> AEFASGSGQSTRYWDCCKPSCAWPGKAAVSQPVYACDANFQRLSDFNVQSGCNGGSAYSCADQTPWAVNDNLAYGFAATSIAGGSESSWCCACYALTFTSGPVAGKTMVVQSTSTGGDLGSNQFDIAMPGGGVGIFNGCSSQFGGLP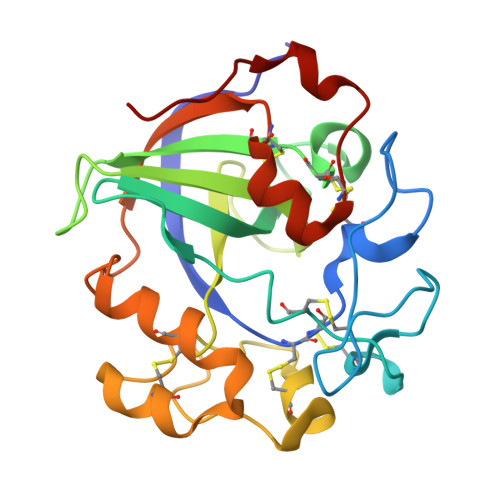GAQYGGISSRDQCDSFPAPLKPGCQWRFDWFQNADNPTFTFQQVQCPAEIVARSGCKRNDDSSFPVFTPS> MASGAPPSVDLTSIQWRMPEWVQS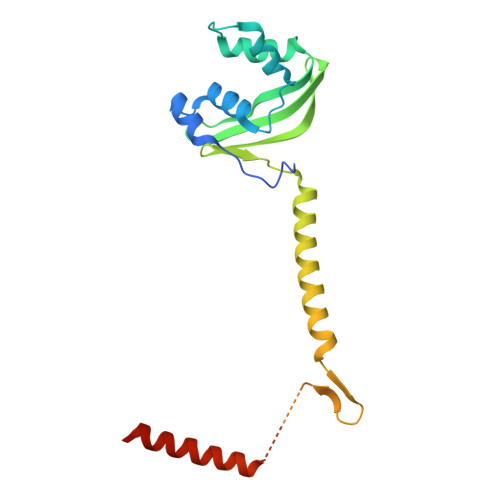MGGLRTENVLEYFSQSPFYSHKSNNEMLKMQSQFNALDLGDLNSQLKRLTGIQFVIIHERPPFLWVIQKQNRLNENEVKPLTVYFVCNENIYMAPNAYTLLATRMLNATYCFQKALTKIEKFPQYNPQEGYTYPKLSNDNLEVDHSNTNEPADENKNQSIENADYSFSPEDFSVVRAFMQSLHSSKEAPDVK>MEGLAGYVYKAASEGKVLTLAALLLNRSESDIRYLLGYVSQQGGQRSTPLIIAARNGHAKVVRLLLEHYRVQTQQTGTVRFDGYVIDGATALWCAAGAGHFEVVKLLVSHGANVNHTTVTNSTPL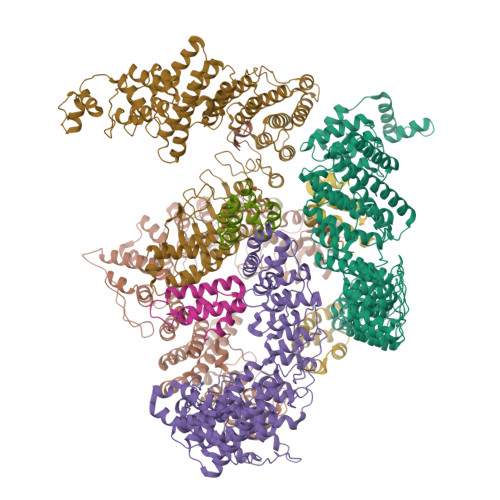RAACFDGRLDIVKYLVENNANISIANKYDNTCLMIAAYKGHTDVVRYLLEQRADPNAKAHCGATALHFAAEAGHIDIVKELIKWRAAIVVNGHGMTPLKVAAESCKADVVELLLSHADCDRRSRIEALELLGASFANDRENYDIIKTYHYLYLAMLERFQDGDNILEKEVLPPIHAYGNRTECRNPQELESIRQDRDALHMEGLIVRERILGADNIDVSHPIIYRGAVYADNMEFEQCIKLWLHALHLRQKGNRNTHKDLLRFAQVFSQMIHLNETVKAPDIECVLRCSVLEIEQSMNRVKNISDADVHNAMDNYECNLYTFLYLVCISTKTQCSEEDQCKINKQIYNLIHLDPRTREGFTLLHLAVNSNTPVDDFHTNDVCSFPNALVTKLLLDCGAEVNAVDNEGNSALHIIVQYNRPISDFLTLHSIIISLVEAGAHTDMTNKQNKTPLDKSTTGVSEILLKTQMKMSLKCLAARAVRANDINYQDQIPRTLEEFVGFH[4x];>DRKRRSDPNFKNRLRERRKKQKLAKERAGLSKLPDLKDAEAVQKFFLEEIQLGEELLAQGEYEKGVDHLTNAIAVCGQPQQLLQVLQQTLPPPVFQMLLTKLPTISQRIVSAQSLAEDDVE[5x]EcFrmR is a member of the CsoR/RcnR family of transcriptional repressors. Therefore, the in vivo and in vitro data showed that EcFrmR is a repressor of frmRAB expression that responds directly to formaldehyde by disassociation of the Pfrm–EcFrmR complex, allowing the expression of the formaldehyde detoxification system. Thus, like other members of the CsoR/RcnR family, EcFrmR is a homotetramer. In vivo and in vitro data show that EcFrmR senses formaldehyde directly, with no metal-dependence, via the formation of inter-subunit methylene bridges between adjacent Pro2 and Cys35 residues.

Like other members of the CsoR/RcnR family, EcFrmR oligomerizes to form a disc-like tetramer, constructed from two homodimers, each of which forms one face of the disc. Each subunit consists of three helices (α1, residues 2–30; α2, residues 35–68; and α3, residues 73–91), linked by two short loops (L1, residues 31–34; and L2, residues 69–72), that are arranged as a flattened S-shape. The formaldehyde-exposed EcFrmR tetramer is asymmetric. One face of the tetramer (A/B face) is comprised of an unmodified homodimer with electron density visible for residues Lys9-Lys91 of both polypeptides with a disordered N-terminal region (residues Pro2-Lys8). In contrast to the A/B face, clear electron density is present for residues Pro2-Lys8 of both subunits on the A′/B′ face, resulting in an ordered extension to the N-terminal region of α1. The Pro2′-N atom is located within ~2.5 Å of the Cys35-SG atom of the corresponding subunit on the opposite face of the tetramer. There is extra density between these two atomic positions, indicating the presence of the formaldehyde cross-link, and a methylene bridge (-CH2-), as indicated by the LC-MS data, has been modeled at this location. The crystal structure of EcFrmR reveals both the free and signal-triggered states of the protein. Whilst the position of α3 is similar on both faces of the tetramer, there is a translational movement of α1 and α2 on the A′/B′ face, which slide across the equivalent helices on the opposite face by ~1.5 α-helical turns in response to formation of the methylene bridge. In addition, the C-terminal half of α2 twists and buckles towards α3, which alters the packing of these two helices, generating a 10° off-parallel angle between α3 and α2. This movement changes the overall size and shape of the A′/B′ face, which expands and elongates by ~10 Å on the diagonal in response to formaldehyde (Animation S1).

>MPSTPEEKKKVLTRVRRIRGQIDALERSLEGDAECRAILQQIAAVRGAANGLMAEVLESHIRETFDRNDCYSREVSQSVDDTIELVRAYLK[4x]>GSVESHPVLEKLKAAHSYNPKEFEWNLKSGRVFIIKSYSEDDIHRSIKYSIWCSTEHGNKRLDSAFRCMSSKGPVYLLFSVNGSGHFCGVAEMKSPVDYNTSAGVWSQDKWKGKFDVQWIFVKDVPNNQLRHIRLENNDNKPVTNSRDTQE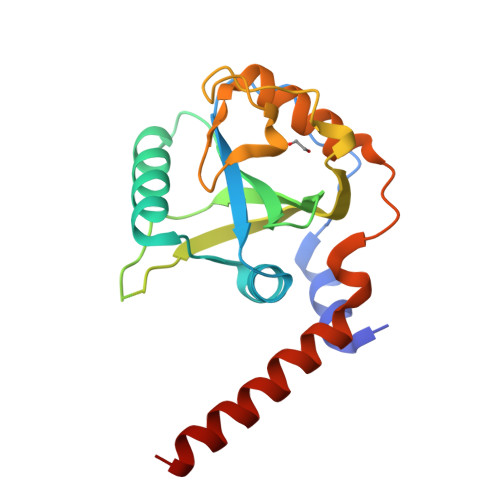VPLEKAKQVLKIISSYKHTTSIFDDFAHYEKRQEEEEVVRKERQSRNKQ[4x]> ARVTVQDAVEKIGNRFDLVLVAARRARQM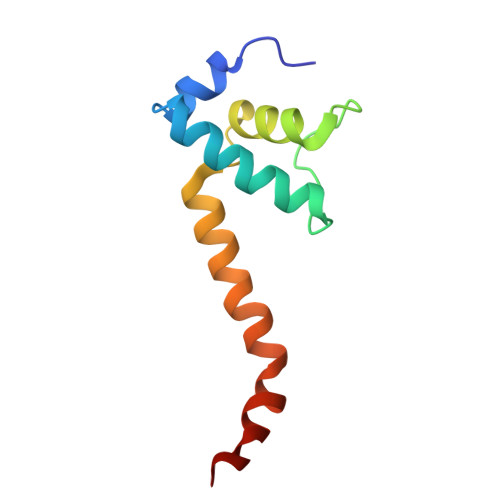QVGGKDPLVPEENDKTTVIALREIEEGLINNQILDVRERQEQQEQEAAELQAVTAIAEGRR>[2x]MYRTHYSSEITEELNGQKVKVAGWVWEVKDLGGIKFLWIRDRDGIVQITAPKKKVDPELFKLIPKLRSEDVV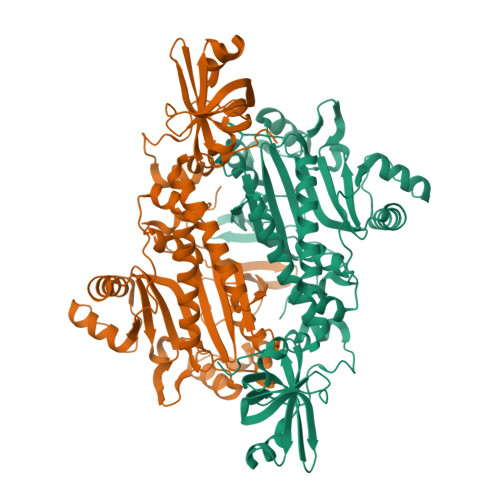AVEGVVNFTPKAKLGFEILPEKIVVLNRAETPLPLDPTGKVKAELDTRLDNRFMDLRRPEVMAIFKIRSSVFKAVRDFFHENGFIEIHTPKIIATATEGGTELFPMKYFEEDAFLAQSPQLYKQIMMASGLDRVYEIAPIFRAEEHNTTRHLNEAWSIDSEMAFIEDEEEVMSFLERLVAHAINYVREHNAKELDILNFELEEPKLPFPRVSYDKALEILGDLGKEIPWGEDIDTEGERLLGKYMMENENAPLYFLYQYPSEAKPFYIMKYDNKPEICRAFDLEYRGVEISSGGQREHRHDILVEQIKEKGLNPESFEFYLKAFRYGMPPHGGFGLGAERLIKQMLDLPNIREVILFPRDRRRLTP CI2 is a small single domain protein of 64 residues, which has been extensively used as a model to understand key concepts of protein folding and stability. L49 and I57 are both part of the folding nucleus in CI2 and very important for the stability of the folded state of CI232. Here, we have applied an efficient in-cell assay in E. coli to select variants of the barley chymotrypsin inhibitor 2 with increased stability. We, therefore, determined the crystal structures of all four CI2 variants in the wild-type to L49I/I57V double mutant cycle.

Instead, the most abundant mutant after selection was I57V which can be made by a single base substitution from the Ala codon. As I57V is more stable than the wild-type this demonstrates the efficiency of the selection system. Relative to the wild-type, I57V is stabilized by ΔΔGf = −2.2 ± 0.1 kJ mol−1. Overall, the structures of L49I, I57V and L49I/I57V are highly similar to the structure of the wild-type with RMSDs for the backbone of 0.16, 0.45 and 0.17 Å. The larger RMSD for I57V is a result of the overhand loop in this structure adopting an alternative conformation compared to the other three structures. The Val at position 57 in I57V and L49I/I57V superimpose, except for the missing δ1 methyl group, with the Ile at position 57 in the wild-type and L49I. Analysis of the pairwise interaction energies at the residue level suggests that much of the stabilizing effect of the I57V mutation originates from an unfavourable interaction between I57 and Q59 that is observed in structures of both the wild-type and L49I.

> MKTEWPELVGKSVEEAKKVILQDKPEAQIIVLPVGTIVTMEYRIDRVRLFVDKLDNVAQVPRVG> NKRAPYWTNTEKMEKRLHAVPAANTVKFRCPAGGNPMPTMRWLKNGKEFKQEHRIGGYKVRNQHWSLIMESVVPSD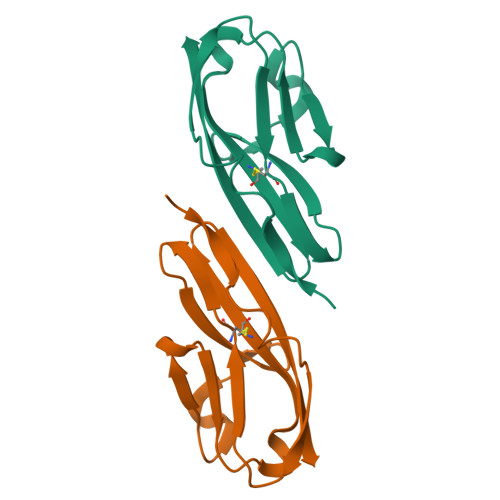KGNYTCVVENEYGSINHTYHLDVV4-[(R)-methylsulfinyl]-2-oxo-6-[3-(trifluoromethoxy)phenyl]-1,2-dihydropyridine-3-carbonitrile 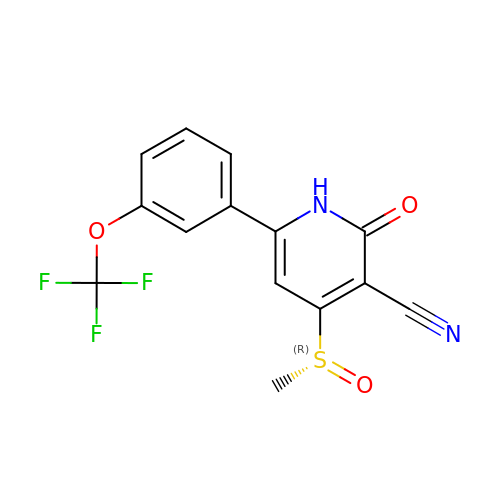| C14 H9 F3 N2 O3 S | LDLFTWUQLJNHAW-HSZRJFAPSA-N> MLRVRCLRGGSRGAEAVHYIGSRLGRTLTGWVQRTFQSTQAATASSRNSCAADDKATEPLPKDCPVSSYNEWDPLEEVIVGRAENACVPPFTIEVKANTYEKYWPFYQKQGGHYFPKDHLKKAVAEIEEMCNILKT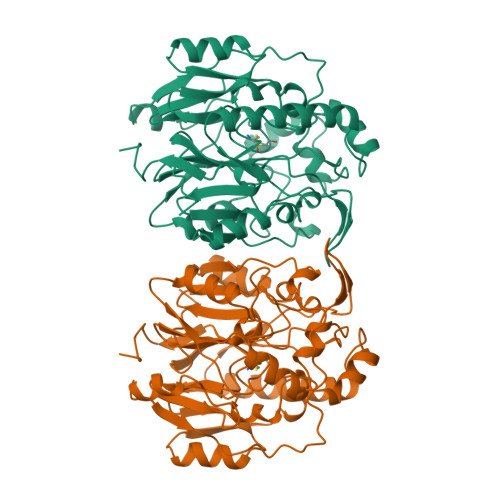EGVTVRRPDPIDWSLKYKTPDFESTGLYSAMPRDILIVVGNEIIEAPMAWRSRFFEYRAYRSIIKDYFHRGAKWTTAPKPTMADELYNQDYPIHSVEDRHKLAAQGKFVTTEFEPCFDAADFIRAGRDIFAQRSQVTNYLGIEWMRRHLAPDYRVHIISFKDPNPMHIDATFNIIGPGIVLSNPDRPCHQIDLFKKAGWTIITPPTPIIPDDHPLWMSSKWLSMNVLMLDEKRVMVDANEVPIQKMFEKLGITTIKVNIRNANSLGGGFHCWTCDVRRRGTLQSYLD> MTPLTPVLSRFWDEPEPWTLETYRRHDGYQGLQRALSMGPDDVIAFVKDSGLRGRGGAGFPTGTKWSFIPQERGDQPAGGPAAKPHYLVINADESEPGTCKDI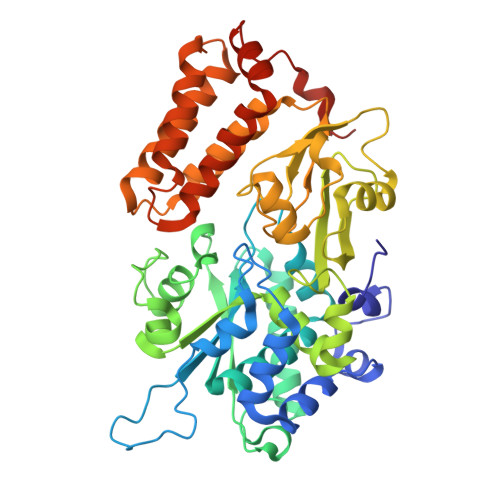PLLLTTPHFLVEGAIIAAYAIRARHAFIYVRGEVLPVLRRLQAAVAEAYAAGYLGTDIMGSGFDLDLIVHAGAGAYICGEETALLDSLEGRRGQPRLRPPFPAVAGLYACPTVVNNVESIASVPPIMVNGVDWFRSMGSEKSPGFTLYSLSGHVTRPGQYEAPLGITLRELLEYAGGVRAGHQLKFWTPGGSSTPLLTAEHLDVPLDYEGMASVGSMLGTKALQIFDETTCVVRAVRRWTQFYAHESCGKCTPCREGTYWLAQIYARLENGAGTEADIDKLLDISDNIFGKSFCALGDGAASPIMSSIKHFRDEYVAHLDGGCPFDPHASTLMATEGAGV> HRQALGERLYPRVQA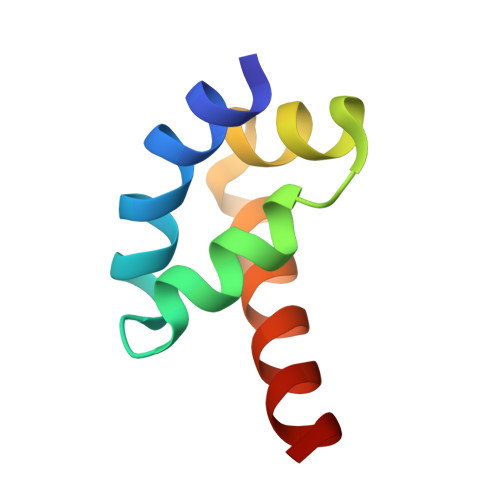MQPAFASKITGMLLELSPAQLLLLLASEDSLRARVDEAMELIIAHG>[2x]MSYYHHHHHHLGSTSLYKKAGMADQERRTFGSYKIEELTIKNDQPNRNTNSSTSQSTENRLSTKKIPLLDDGIFELLNYLIDGT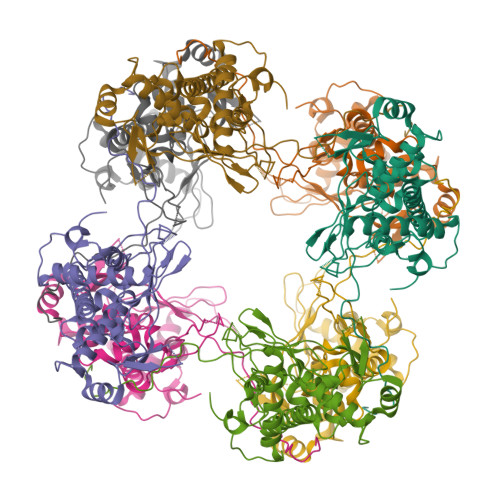NFDKTCYCGFNYSHLPNLERDFNVASIYVRENFELCTENLDLKDYDRQANISVKSPDFTLLLEYTLKPSSETDPTIPENEKEENSKPVTPKVVTPKEEKKTVEMSLLPILNRESEESLSSEILEGEAAVVNVFKMYIKGFLMYLGENPNSYDRQLNIEKYRPLLISIIGYEHLIGTRVPNKEVNHIFYQLATFDNYPFDLLRFQLSSLISTPALIREKIAKEGLFKIITSNTLRGASRQTVLFRGINGSESFLNIKRYRKFKTRIVGNVDCVIKSDFSSLKLDV>[2x]MEEPEEPADSGQSLVPVYIYSPEYVSMCDSLAKIPKRASMVHSLIEAYALHKQMRIVKPKVASMEEMATFHTDAYLQHLQKVSQEGDDDHPDSIEYGLGYNCPATEGIFDYAAAIGGATITAAQCLIDGMCKVAINWSGGW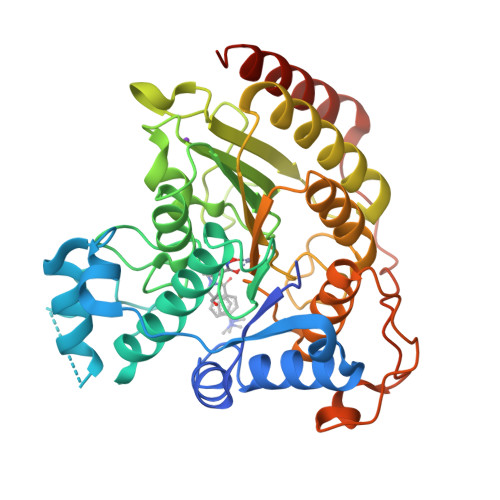HHAKKDEASGFCYLNDAVLGILRLRRKFERILYVDLDLHHGDGVEDAFSFTSKVMTVSLHKFSPGFFPGTGDVSDVGLGKGRYYSVNVPIQDGIQDEKYYQICESVLKEVYQAFNPKAVVLQLGADTIAGDPMCSFNMTPVGIGKCLKYILQWQLATLILGGGGYNLANTARCWTYLTGVILGKTLSSEIPDHEFFTAYGPDYVLEITPSCRPDRNEPHRIQQILNYIKGNLKHVVIEGRSHHHHHH> MAPQIRSRSLAAQEPASVLEEARLRLHVSAVPESLPCREQEFQDIYNFVESKLLDHTGGCMYISGVPGTGKTATVHEVIRCLQQAAQANDVPPFQYIEVNGMKLTEPHQVYVQILQKLTGQKATANHAAELLAKQFCTRGSPQETTVLLVDELDLLWTHKQDIMYNLFDWPTHKEARLVVLAIANTMDLPERIMMNRVSSRLGLTRMCFQPYTYSQLQQILRSRLKHLKAFEDDAIQLVARKVAALSGDARRCLDICRRATEICEFSQQKPDSPGLVTIAHSMEAVDEMFSS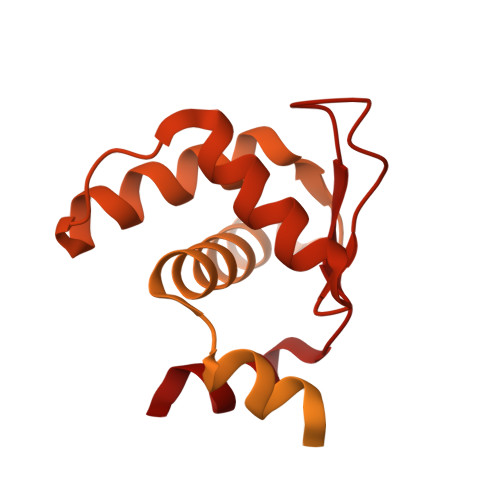SYITAIKNSSVLEQSFLRAILAEFRRSGLEEATFQQIYSQHVALCRMEGLPYPTMSETMAVCSHLGSCRLLLVEPSRNDLLLRVRLNVSQDDVLYALKDE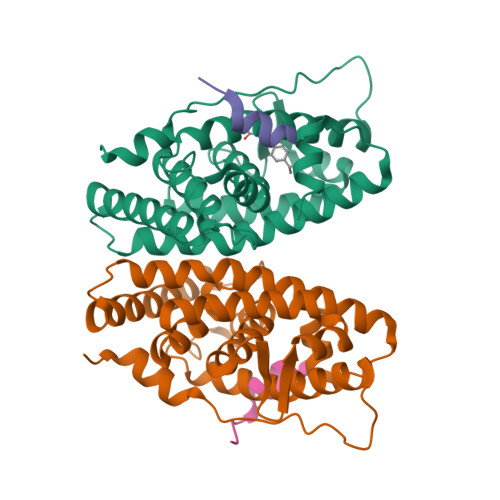>[2x]PAKKPYNKIVSHLLVAEPEKIYAMPDPTVPDSDIKALTTLCDLADRELVVIIGWAKHIPGFSTLSLADQMSLLQSAWMEILILGVVYRSLSFEDELVYADDYIMDEDQSKLAGLLDLNNAILQLVKKYKSMKLEKEEFVTLKAIALANSDSMHIEDVEAVQKLQDVLHEALQDYEAGQHMEDPRRAGKMLMTLPLLRQTSTKAVQHFYNIKLEGKVPMHKLFLEMLEAKV;>LERNNIKQAANNSLLLHLLKSQTIP[2x]> ELDLETLAPYIPMDGEDFQLX;> GSGSPNGQTKPLPALKLALEYIVPCMNKHGICVVDDFLGKETGQQIGDEVRALHDTGKFTDGQLVSQKSDSSKDIRGDKITWIEGKEPGCETIGLLMSSMDDLIRHCNGKLGSYKINGRTKAMVACYPGNGTGYVRHVDNPNGDGRCVTCIYYLNKDWDAKVSGGILRIFPEGKAQFADIEPKFDRLLFFWSDRRNPHEVQPAYATRYAITVWYFDADERARAKVKYLTGEKGVRVELNKPSDSVGKDVF

The EPAS1 gene encodes for the hypoxia-inducible factor 2 alpha (HIF2α), an essential component of the cellular oxygen-sensing pathway in humans. Under oxygenated conditions, HIFα subunits are hydroxylated by prolyl-hydroxylase enzymes (PHDs) at two conserved proline residues within the oxygen-dependent degradation domain (ODD). Hydroxylated HIFα is recognized by the von Hippel-Lindau tumor suppressor protein (pVHL), the substrate receptor of an E3 ubiquitin ligase comprised of Elongin B, Elongin C, Cullin-2, and Rbx1 that polyubiquitylates hydroxylated HIFα subunits targeting them for destruction by the 26S proteasome. Pacak–Zhuang syndrome mutations are concentrated in the HIF2α sequence to the residues in proximity to P531 within the C-terminal ODD (CODD) region.

We crystalized the PHD2/HIF2α-CODD complex in the presence of FeSO4 and NOG to stabilize the interaction and prevent reaction turnover. Well-defined electron density was observed for all 20 amino acids of the HIF2α-CODD peptide allowing for a detailed analysis of the binding interface. The HIF2α-CODD peptide is observed to fit into a cleft in the PHD2 surface with P531 positioned nearby to the coordinated Fe2+ atom in the PHD2 active site and the PHD2 inhibitor NOG is observed to coordinate the Fe2+ atom. The loop containing V241-K244 of PHD2 wraps around the top of the peptide, enclosing HIF2α P531 in the PHD2 active site. Overall HIF2α-CODD binds to PHD2 in a similar manner as HIF1α-CODD (PDB: 5L9B16). The main structural differences in PHD2 between the two structures are localized to the loop containing K244 and the end of the helix around Y403, which are both slightly repositioned relative to the PHD2/HIF1α-CODD complex structure to accommodate the HIF2α-CODD. In our HIF2α-CODD structure, the backbone carbonyl group of the corresponding D525 residue forms a hydrogen bond with the T528 side chain disrupting the helix structure and directing the D525 side chain away from PHD2 K244, not allowing the formation of a salt bridge. The presence of an additional glycine residue (i.e., G537) in the middle of the CODD sequence of HIF2α relative to HIF1α results in a reorganization in the surrounding residues that maintains the side chain interactions previously observed in the PHD2/HIF1α-CODD structure with some altered distances between the corresponding residues to accommodate the additional glycine residue. This adjustment of the positions of side chains results in an overall increase in the distance between the sulfur atom of HIF2α M535 and PHD2 Y403 by 0.6 Å relative to the corresponding HIF1α M568 and PHD2 Y403. There is a sharp increase in atomic B-factor values in residues P534-D539 relative to the rest of the peptide indicating that this segment of the peptide has increased flexibility, likely due to the reduced contact with PHD2.> MSSAEEEVHHDLEIQEVDAGSQEKATIPVNKLKKGGYVLIEGRPCRVVDITKSKT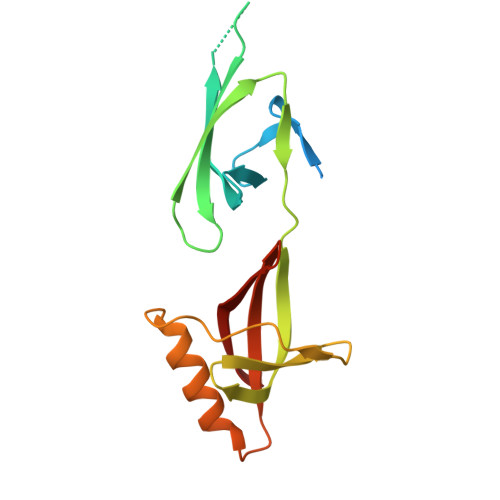GKHGHAKAGIAGTDLFTGRRYETHLPTSHEIEVPFVDRSDYGLINIDDGHTQLLTLDGTLREDVDLPPEGNEMRQRVIDLFNVCVNTNDQVVVTVLSSNGENLIVDCKKSTN>HHHHHHSSGLVPRGSHMLLTADTVLTGTELLRPGWLEIASDRVVAVGAGAPPAQADRNLGAATVVPGFVDTHLHGGGGGNFSAATDDETARAVALHRAHGSTTLVASLVTAGPEDLLRQVSGLARQVRAGLIDGIHLEGPWLSTLRCGAHQPVLMRDPDPGEIGRVLDAGEGTVRMVTIAPERDGALAAIAQLVNAGVVAAVGHTEATYDQTRAAIDAGATVGTHLFNAMRPIDRREPGP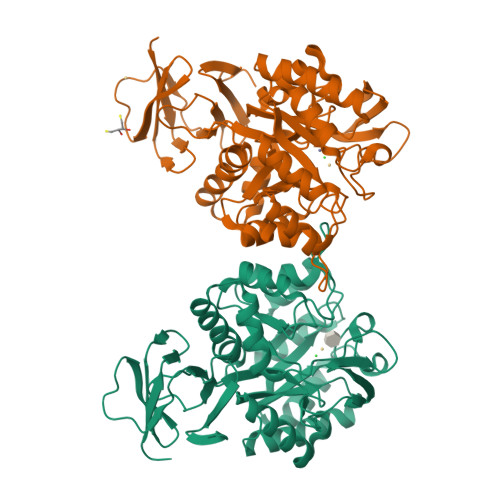AVALTEDSRVTVEMIVDGVHVAPAIYRHITQTVGPERLSLITAAMAATGMSDGVYRLGPLDIDVVAGVARVAGTDTIAGSTATMEQVFRLAVAHCGLPRDDALSLAVRQACVNPARALGLPAAGLAAGARADLVVLDHDLAVTAVMRAGEWVVTPGAAHTV[2x]> MRNLMRCLIMIKSLIKGVDMS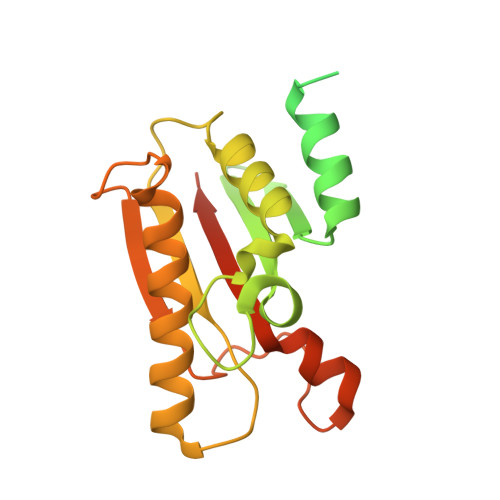RKLAKTRILGYGLMICFLAGCFHPPYNNFQPDRRAVKRVGVDTGIGAVAGAIASGTASGTLIGAAAGGTVGLVASIYRDSKRKIIRDLQKQDIQYVEYGDTRTLIIPTDKYFMFSSPRLNEICYPGLNNVIRLLNFYPQSTIYVAGFTDNVGSRSHKRKLSQAQAETMMTFLWANGIAAKRLKAEGYGDKNAISDNAIIHGSAQNRRIEIQWFTSPAQPPQPQMAYVK>ELPNYLVTLPARLNFPSVQKVCLDLSPGYSDVKFTVTLETKDKTQKLLEYSGLKKRHLHCISFLVPPPAGGTEEVATIRVSGVGNNISFEEKKKVLIQRQGNGTFVQTDKPLYTPGQQVYFRIVTMDSNFVPVNDKYSMVELQDPNSNRIAQWLEVVPEQGIVDLSFQLAPEAMLGTYTVAVAEGKTFGTFSVEEYVLPKFKVEVVEPKELSTVQESFLVKICCRYTYGKPMLGAVQVSVCQKANTYWYREVEREQLPDKCRNLSGQTDKTGCFSAPVDMATFDLIGYAYSHQINIVATVVEEGTGVEANATQNIYISPQMGSMTFEDTSNFYHPNFPFSGKIRVRGHDDSFLKNHLVFLVIYGTNGTFNQTLVTDNNGLAPFTLETSGWNGTDVSLEGKFQMEDLVYNPEQVPRYYQNAYLHLRPFYSTTRSFLGIHRLNGPLKCGQPQEVLVDYYIDPADASPDQEISFSYYLIGKGSLVMEGQKHLNSKKKGLKASFSLSLTFTSRLAPDPSLVIYAIFPSGGVVADKIQFSVEMCFDNQVSLGFSPSQQLPGAEVELQLQAAPGSLCALRAVDESVLLLRPDRELSNRSVYGMFPFWYGHYPYQVAEYDQCPVSGPWDFPQPLIDPMPQGHSSQRSIIWRPSFSEGTDLFSFFRDVGLKILSNAKIKKPVDCSHRSPEYSTAMGAGGGHPEAFESSTPLHQAEDSQVRQYFPETWLWDLFPIGNSGKEAVHVTVPDAITEWKAMSFCTSQSRGFGLSPTVGLTAFKPFFVDLTLPYSVVRGESFRLTATIFNYLKDCIRVQTDLAKSHEYQLESWADSQTSSCLCADDAKTHHWNITAVKLGHINFTISTKILDSNEPCGGQKGFVPQKGRSDTLIKPVLVKPEGVLVEKTHSSLLCPKGKVASESVSLELPVDIVPDSTKAYVTVLGDIMGTALQNLDGLVQMPSGCGEQNMVLFAPIIYVLQYLEKAGLLTEEIRSRAVGFLEIGYQKELMYKHSNGSYSAFGERDGNGNTWLTAFVTKCFGQAQKFIFIDPKNIQDALKWMAGNQLPSGCYANVGNLLHTAMKGGVDDEVSLTAYVTAALLEMGKDVDDPMVSQGLRCLKNSATSTTNLYTQALLAYIFSLAGEMDIRNILLKQLDQQAIISGESIYWSQKPTPSSNASPWSEPAAVDVELTAYALLAQLTKPSLTQKEIAKATSIVAWLAKQHNAYGGFSSTQDTVVALQALAKYATTAYMPSEEINLVVKS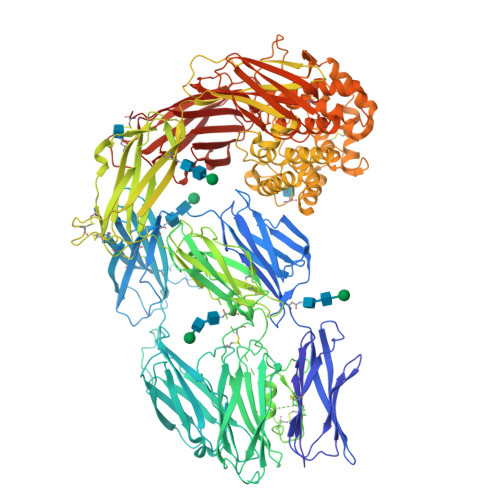TENFQRTFNIQSVNRLVFQQDTLPNVPGMYTLEASGQGCVYVQTVLRYNILPPTNMKTFSLSVEIGKARCEQPTSPRSLTLTIHTSYVGSRSSSNMAIVEVKMLSGFSPMEGTNQLLLQQPLVKKVEFGTDTLNIYLDELIKNTQTYTFTISQSVLVTNLKPATIKVYDYYLPDEQATIQYSDPCE[2x]> MQQLNENKIIKLLRDNI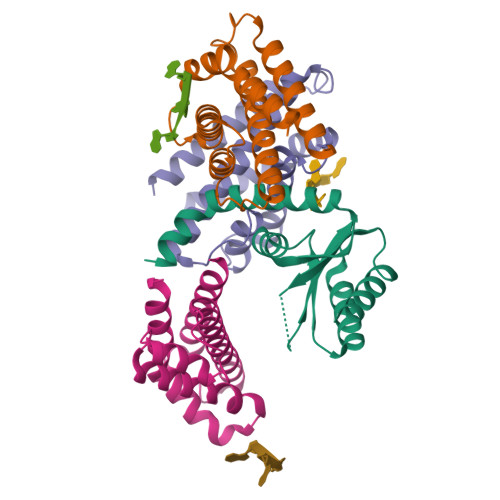PKLQLIYLFGSYSQGTQHRNSDIDIAVLAADTLDNIARWELAQKLASALDSDVDLVDLRSASTVLCQQVVTQGKQLWGTQQDDELFAVKTISMYQHLQAERQAIIDDVMANTAAKAHRGESL;>MNDIIINKIATIKRCIKRIQQVYGDGSQFKQDFTLQDSVILNLQRCCEACIDIANHINRQQQLGIPQSSRDSFTLLAQNNLITQPLSDNLKKMVGLRNIAVHDYQELNLDIVVHVVQHHLEDFEQFIDVIKAE[3x]>GPGSMEIRDAVAVVTGGASGLGLATTKRLLDAGAQVVVLDIRGEDVVADLGDRARFAAADVTDEAAVASALDLAETMGTLRIVVNCAGTGNAIRVLSRDGVFSLAAFRK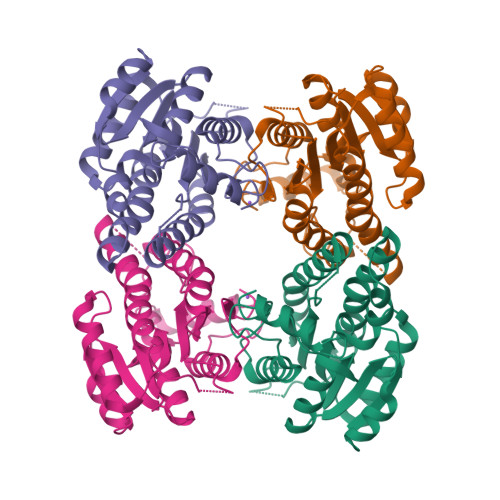IVDINLVGSFNVLRLAAERIAKTEPVGPNAEERGVIINTASVAAFDGQIGQAAYSASKGGVVGMTLPIARDLASHRIRVMTIAPGLFDTPLLASLPEEARASLGKQVPHPSRLGNPDEYGALAVHIIENPMLNGEVIRLDGAIRMAPR[2x]4-[(7-CHLOROQUINOLIN-4-YL)AMINO]-2-[(DIETHYLAMINO)METHYL]PHENOL | C20 H22 Cl N3 O | 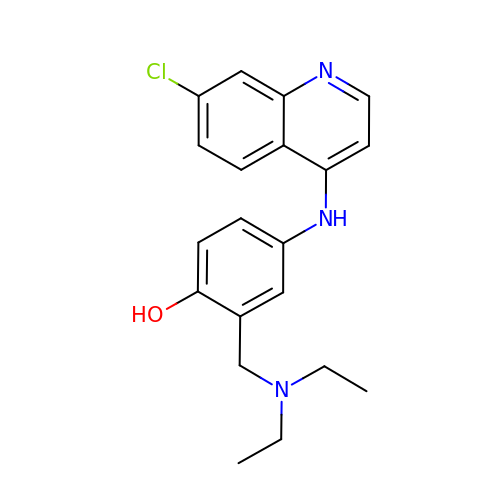OVCDSSHSILBFBN-UHFFFAOYSA-N>MSEFRIHHDVNELISLLHVFGLEGADVYIDLLQKNRTPYVTTSVSTHSAKVKIAEFSRTPDDFLKKYEELKSKNTRNLDPLVYLLSKLIEDKETLQYLQQNAKDKAELATSSVTSVSLPIAPNTSKISMQELEELRRQLETATVAVSCSHQPVEVLRKFLRDKLNKKHTGHPVPVFPSWVYERPALTGDFMSFSNPSTDVTVSIGTLPLPSQETCLVEDLLYILIGVDGRYISVQPLVGRQSRSFSVEQNLDSSVKELVNRILPVATNYSTVTRFVEENSSFEYGQVNHALGAAMRTLGKEYMILISQLEHLQRQGLLSLQKLWFYIQPTLRTMEVLASIATSLNKGECFGGATLSLLHDRTFGYTGDSQAQELCLYLTKAASAPYFDILERWIYRGIINDPYSEFMVEEHELQKEKIQEDYNDKYWDQRYTIVQQQIPSFLQKVADKILSTGKYLNVVRECGHDVTCPDAKEITYTLKEQAYVERIEKAYNYASKVLLDFLMEEEELVAHLRSIKHYFLMDQGDFFVHFMDLTEEELKKPVDDIIPTRLEALLELALRMSTANTDPFKDDLKIELMPHDLITQLLRVLAIETHQEKALINSDPTELALSGLESFSFDYIVKWPLSLIINRKALTRYQMLFRHMFYCKHVERLLCNVWISNKTAKQFSLHSAKWFAGAFTLRQRMLNFVQNIQYYMMFEVMEPTWHILEKNLKSASNIDDVLSHHTSFLDNCLKDCMLTNPELLKIFSKLMSVCVMFTNCLQRFTQSMQVQTEMEHLTLEHGTMMGPPTQCERTEEALKKKLTSKYLEEHIDKFPSSFGFESTINNFDSNFSAHLMDLLDKLSMYSTSDCEHSMINIIYRLDFNGFYTERLKQLSSERNQKSAPLLGPAQHAVSTK[4x];>[9x]MAVPDQKSPNVLLQNLCCRILGKGEADVAQQFQYAVRVIGSNFAPTVERDEFLVTEKIKKEFVRQRREADGALFSELHRKLQSQGVLKNRWSILYLLLSLSEDPRKQPNKTSSFAALFAQALPRDAHSTPYYYARPQSLPLSYQDRNVQCAQNAASIGSSGISSIGMYALNGPTPQSIIQGQSNQTPNMGDALRQQLGSRLAWTLAAGQQPSQQSTTTKGLPNTVSRNVPRTRREGDSSGSVEITETSLVRDLLYVFQGIDGKFVKMCNSENCYKVDGKVAVSKSLKDITSKLSELGWLHNKIKKYTDQRSLDRAFGLVGQSFCAALHQELKEYYRLLSVLHSQLQVEDDQGVNLGVESSLTLRRLLVWTFDPKIRLKTLAALVDHCQGRKGGELASAVHAYTKTGDPYMRSLVQHILGLVAYPILNFLYRWIYDGELEDTYHEFFVASDPVVKTDRLWHDKYSLRKSMIPSFMTMDQSRKVLLIGKSINFLHQVCHDQTPASKAMAVGKSAESPKDAAELFTDLENAFQTKIDAAYFDTSKYLLDVLNKNYNLLEHMQAMRRYLLLGQGDFIRHLMDLLKPELVRPATTLYQHNLTGILETAVRATNAQFDNPEILKRLDVRLLEVSPGDTGWDVFSLDYHVDGPIATVFTRECMSHYLRVFNFLWRAKRMEYILTDIWKGHMCNAKLLKGMPELSGVLHQCHILASEMVHFIHQMQYYITFEVLECSWDELWNKVLKAQDLDHIIAAHDVFLDTIISRCLLDSESRALLNQLRAVFDQIIEFQNAQDALYRAALEELQQRLQFEERKKERESEGEWGVTAAEEDVENKRIQEFQESIPKMRSQLRILTHFYQGIVQQFLVLLTTSTDESLRFLSFRLDFNEHYKAREPRLRVSMGTRGRRSFHV;>MIHELLLALSGYPGSIFTWNKRTGLQVSQDIPFLHPGETSVLNRLCKLGTDYIRFTEFIEQYTGHVQQQDHHPSQQGQVGLHGIYLRAFCRGLDSILQPYRQALLDLEQEFLADPHLSISHINYSLDQFHLLFPSIMVVVEQIKSQKIHGCQILETVYKHSCGGLPPVRSALEKTLAVCHGVMYKQLSAWMLHGLLLDQYEEFFVRQGSSSGNLAAAFEEEEDDLGIGGLTGKQLRELQDLRLIEEENMLAPSLKQFSLRAEMLPSYIPVRVAEKILFVGESVQMFENQNVNMSRTGSILKNQEDTFAAELHRLKQQPLFSLVDFESVLDRIRSTVAEHLWKLMVEESDLLGQLKIIKDFYLLGRGELFQAFIDVAQNMLKTPPTAVTEHDVNVAFQLSAHKVLLDDDNLLPLLNLTIDYHGKEHKDTSQPREGPFRDMSPREAPTSGWAALGLSYKVQWPLHILFTPAVLEKYNVVFKYLLSVRRVQSELQHCWALQMQRKHLESNKTDAIKWRLQNHMAFLVDNLQYYLQVDVLESQFSQLLQQINSTRDFESIRLAHDHFLSNLLAQSFILLKPVFHCLNEILELCHSFCSLVSQNLGPLDERGAGQLDILVKGFSCQSSLLFRILSSVRNHQINPDLAQLLLRLDYNKYYTQAGGTLGSFGL[2x];> MAHWTRFERDQEGDIKKLVSLMSGIQDDQDGNFQQALQFAWSNFRFHRYLDVSSHTVLRTLEGIFEKLVVHSDLEKAESWKRLTEEFLLLPLPNTEGTKTDSHFAVLSLLLCLSDSPSNHDYTEKPRKKENDEQEPFDWGKYLREGEDIEFSPDADTPEWSEASEEEDAQEPPSREDSGIQVDRTPLEDPEKKGAPPLVSWKVGEPDARSWLEQHIVHQYWTSRAPRFSHSSHLHSNLSAIWDQHLYTTDPLYTPDDKTIVTETQVIRETLWLLSGVKKLLIFQLNDGKVNVRNDIIVTHMTQNCLRSVLEQIAAYGQVVFRLQKFIDEITGHGSEVPLPGTLPTAKKTTEAPFRTYQAFMWALYKYFISFKEELTEIEKCIINKDETVTLAIVLDKLAPRLAQLKVLHRVFSTGIAEVPPDTRNVVRASHLLNTLYKAILDYDNVGEASEQTVSLLFCLWVETVRPYLEIVDEWIVHGNLFDPAKEFIIQRNKDVPFNHRDFWYATYTLYSVSEKTENEDKMSDNASASSGSDQAPAGRQHTMVSFLKPVLKQIIMAGKSMQLLKNLKCRTALQQDSSRDSDRKSLYTLFLESVQSRLQHGNDSVPDIITEQQVNKLSLIKMQSIVAKHLELDEVHDPLLAINFVRLYLEQSDFLETFTCNEVCVDRSSESVTCQSFELTLRSCLYPHIGKQYLECCGNLMYTLKKDYRLVEYLQAMRNFFLLEAGDTMYDFYTPIFDKIREKEPWLNLSYLNVQIQEAVGQRYPDDSTRLSVSFESVDLAKKKLPVHTLDGLILSYKVPWPVDIVISSECQKIYNQVFLLLLLIKWAKYSLDVLQFNELGNASENESTKEGATVEPFPLPPLTSPSEPKGQQIHRMFLLRVKLMHFVNSLHNYLMTRILHSTGLEFQHQVEEAKDLDQLIKIHYRYLSTIHDRCLLREKVSSVKEAIMKVLNVVLMFADRWHAGLGAWKKESIVKMESDFTNCHKFLVKVLNKAVCRGSFPHLESLALSLMAGMEQS;> MDSITKLFGDLCESHMVGFPWRTALNSRKHSKNRTKQTLKKLAYDTLFVHLFQDEARKLQPNCTRLPVKNKIIMLSFNLRICGMSSEADRLEELVEYLEQSNGIQISDLHAVLELLVELSGTGPPQLLPPKRDYFKNNKYVGRNVKYQGYDYYDVQVFEADLGTTVAYQELEISTTIQRTLQIMEAAPGTGLPALSFFSQNDLSTDKFEKETRGSLFGALVHSRTNDMDIKLDMPPVPENADLSGLAIKVPQSIDQSEDEGFQSASNMTPDSQSEPSMTPDIDVWEAVLTYGPSKRRCWERIGCPPGKREEPYVTEAGREAFDKLYKLHEGGLQILSATTLQPQLVLLEETDLVKAVLNVLIGVVSSTFSYNQALQSFAVKQGVYISGTSPDNVSSLLTQVAEYGTYYTRLSHFSLLTVLDSSHSNGLVFQAFTSGLRKYLQYYRACVLSTPASLTLLTISFLFRKLGRQLRYLAELCCIGTLVTSATRGISTAFPTGVKLLSYLYKEALENSSNENYPVLLSLLKTSCEPYTRFIYDWVYSGVFRDVCGEFMIQVNEDYLGFRDKRYWTHGYVLISKEVEDCVPVFLKHVANEIYICGKTINLLKLCCPKHYICWSDIPVPRISVTFSLEELKEMEKDCAVYVARMERIARHSCISKEQKALQTEIARQELIIQARETTEKVFETFKDRKLAEKLSLDTKKRELFQKLKDQYEKEQERRLTTKQEEADDDFSYAREIRDREKRLKALEEELELKTRQELIEHYSRLSEEATRKEQRALWKLQRHKLETIRLKFFLEEQKRMQDLVANFPVDICEENLGVLPDGEISHQTDNTNDAGLGNIENEKSVPEQHALHNNNDEVYTAQNCISKSESLCVDVTLPTENVHSQTSNASVLGVPSFDSNLCTPDVDIIDFLPTLPSENQEVAVVQSLVDDALISIGSDLNTDTKDKESLCALKSDLQESSTGSEYDFKTILKPIACTQVSQGHIKIGEYSSNVQPARPRWSTHGHSSDSNIKIGNYVSDINVHQPKHSQHGHSSDSNINISDHMSDVEPRLPRLNLHGHISTGHIKVGEYASDVEPSTPRHSVHGHASQGNIKIGENVSDVKLSRPRWNIHGHVSDANIKIGENTSEIAPLRPRWNIHGHASQSHIKIGELVSDIEPSQPRRTPFGHPSQSSIPIGDQPVEKYAQKSESEVHSSNSTIQHLLYSNIPDKNKDTGGTLTDSPVPVPDQGNSNDDTEKRSSTLEQRVQAADSVCDGEASPNTAQSLPCMSDTLDFGTNGEENVGNDDHTWEKQQEYLKGLAEKYCLEKYQDSYELMSHPPVLHLYSNVMPNRFSFPTDSDIKSATDETTVQLIELLSLPVLMKYSVTAPMVSHVYLVNKAIVDYYFVELKMERHFEAMRHFLLMEDGEFAQSLSDMLFEKLGSGQTPSELLNPLVLNSILNKALQYSLHGDSSLASNLTFALKYLPEVFTPTAPDALSCLELKYKVDWPLNIVITDTCMNKYSRIFSFLLQLKHMVWTLRDVWFHLKRTALVNQASNSVQYRQLQL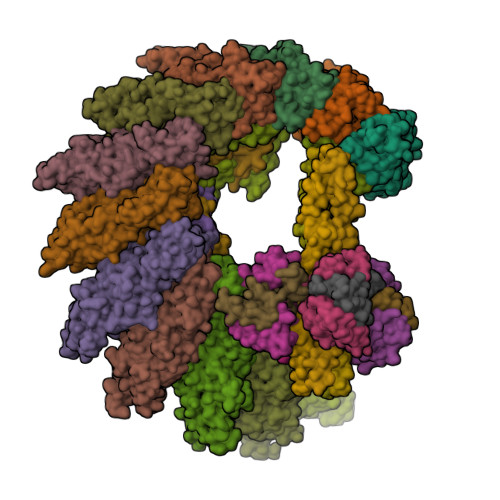YRHEMQHFVKVIQGYIANQILHVTWCEFRNKLSAVSNLEEIYKTHADYLNKALFRGLLTEKAAPLMNIIHSIFSLILKFRLQLISQSWICDTGKQMAVHPNFGLMQQSYNTFKYYSDFLFEVVSKLVNRGYQPHLEDFLLRINFNSYYKQS;>[4x]MESRGGGGRVRLPGTTMQDNIRFVSAGDDVKIWDYSSMTTVEQFNPHSASHPVSSLCWSSNNHFLVTASGSGDKIVVSSCKSKPVPLLELAEGKKQTCVNLNSSSQYVVSGGLDNTVNIWDLKSKRLHRSLKDHKDEVTCVTFNANDCYVASGSMSGEIILHNVTTNLSSTPFGHGSSQPIRHLKYSYVKKSLLGTVSDSGSVTLWDANSQNPYHVFESAHKAPASGICFSPVNDLLLVTVGLDKRIICYDVSSKILLQTVVAESPLTAVDFMPDGATLAVGSSRGKIYLYDLRMLSSPVKTVSAHKTSVQCIQFQHSNIYKSSKGPSSKSSILSTAVNKKPSTKTAAGGTQSANITKDLPPSAISSLPQPVMPVDSKVLRVNDDKSGFPRSTSLDIIPSKETDFAKTSDYKSIDSFGRSSLGDIFSPVRDDASHFRGAEDLSCKGNDLDYLPQFSTIPSSRRNPVGANTQGIHGSPLHLIIESPIKEEDESQDSELKTRKPQLLKQDFRESSSKPASVDQNNLNNSPINSVTRTPEAIEKTGHQILSQLKSDVPAHGTKIASPKVAATMSTQLASSLSEKIADTLASDRTGAPLTAIQINFIKNMIEETLDDFREACHRDIVNLQVEMIKQFHIQSSEIQMLLERYSLNESLVSEIEKLREENKRLRANF;>MANASGNMSAVRETMDVLLEISRLLNTGLDMETLSICVRLCEQGINPEALSSVIKELRRASDTLKASESTAS[6x]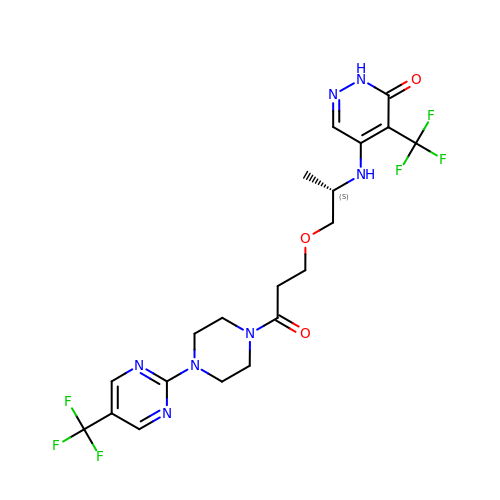5-{[(2S)-1-(3-oxo-3-{4-[5-(trifluoromethyl)pyrimidin-2-yl]piperazin-1-yl}propoxy)propan-2-yl]amino}-4-(trifluoromethyl)pyridazin-3(2H)-one | C20 H23 F6 N7 O3 | UQZCQKXJAXKZQH-LBPRGKRZSA-N> ALKPLKTWSHLAGNRRRPSEYEVVSTNLHYFTDNPERPWELDSNLPMQTWYKKYCFDSPLKHDDWNAFRDPDQL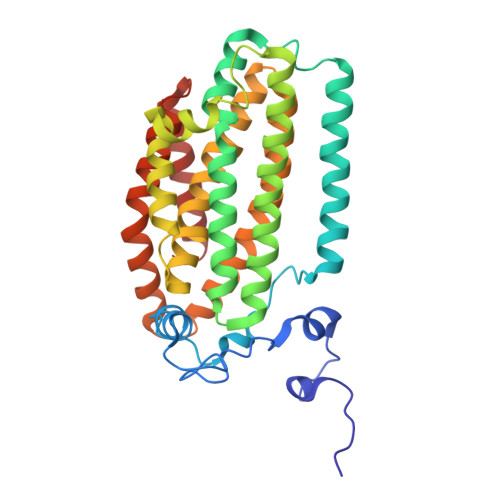VYRTYNLLQDGQESYVQGLFDQLNDRGHDQMLTREWVETLARFYTPARYLFHALQMGSVYIHQIAPASTITNCATYETADHLRWLTHTAYRTRELANCYPDVGFGKRERDVWENDPAWQGFRELIEKALIAWDWGEAFTAINLVTKPAVEEALLQQLGSLAQSEGDTLLGLLAQAQKRDAERHRRWSSALVKMALEKEGNREVLQKWVAKWEPLADKAIEAYCSALPDGENAIVEAKSASRYVRQMMGL Ribonucleotide reductases (RNRs) are essential enzymes that use radical-based chemistry to catalyze the reduction of ribonucleotides to deoxyribonucleotides. Anaerobic class III RNRs (NrdDs), the subject of this study, use an oxygen-sensitive glycyl radical cofactor and are members of the glycyl radical enzyme (GRE) family. The activity of NrdD enzymes can be allosterically up-regulated by ATP and down-regulated by dATP. We find that StNrdD’s regulatory “cone” domains adopt markedly different conformations depending on whether the activator ATP or the inhibitor dATP is bound and that these different conformations alternatively position an “active site flap” toward the active site (ATP-bound) or away (dATP-bound).

An x-ray structure of StNrdD bound to dATP was determined to 2.6-Å resolution by soaking WT-StNrdD crystals in 10 mM CTP and 10 mM dATP. Two dATP molecules are bound in the cone domain of StNrdD as was observed recently for PcNrdD and discussed in detail below. We find one dATP molecule bound in the canonical allosteric activity site (site 1) as first identified in EcRNR. The most unexpected feature of this dATP-bound StNrdD crystal structure is the asymmetric arrangement of the cone domains compared to the dimeric protein core. The cone domains, which form an antiparallel dimeric unit, are tilted so they contact only one side of the core fold, the side of the NrdD dimer that contains the opening to the chain B active site within the 10-stranded barrel. The chain B cone domain sits close to the top of the chain B barrel, not only burying a relatively large surface area near the barrel edge (525 Å2) but also making contacts with chain A across a chain A–chain B interface (left side of dimer in Fig. 2B). We find that the chain B cone domain is near the opening of the chain B barrel but the cone domain is rotated, such that the C terminus end of helix 4 is pointing away from the barrel opening (~180° away), pulling the connector in the opposite direction from the active site. Here, the C terminus of the cone domain helix 4 is pointing in the correct direction toward the chain A active site, but the chain A cone domain is sitting on the opposite side of the NrdD dimer from the barrel opening and is thus too far away for the connector to reach the active site (right). The asymmetry of the dATP-bound structure is therefore part of the mechanism of inhibition.

>[2x]MIILEKERVTVNPDIKVIKRDGRMVTFDSSKIYEAILKASETITPITPLIETKLEGIANRVVAEINDRFSHNIKIYEIQSIVEHELLEANEYAIAQEYINYRTKRDFERSQATDINFTINKLVNKDQAVVHENANKDSDLYNTQRDLTAGIVGKSVGLKMLPPHVANAHQKGDIHFHDLDYSPYTPMTNCCLIDFKGMLANGFKIGNAEVESPKSIQTATAQISQIIANVASSQYGGCTADRIDEFLAPYAELNYKKHLADAKEWVTEEKQEDYARAKTRKDIYDAMQSLEYEINTLFTSNGQTPFTSLGFGLGTNWFEREIQKAILQVRILGLGSEHRTAIFPKLIFTLKRGLNLEPNSPNYDIKQLALECATKRMYPDVLSYDKIIELTGSFKAPMGCRSFLQGWKDENGVEVNSGRMNLGVVTLNLPRIALESKGDQDKFWEIFEERMGIAKDALVYRVERVKEATPANAPILYQYGAFGQRLRKCDSVDQLFKHRRATVSLGYIGLYEVASVFYGSDWETNLEAKTFTLNIVKAMKNACESWSDEYDYHFSVYSTPSESLTDRFCRLDTEKFGVVTDITDKEYYTNSFHYDVRKNPTPFEKLEFEKDYPEAGATGGFIHYCEYPVLQQNPKALEAVWDFAYDRVGYLGTNTPIDKCYKCDFEGDFTPTERGFMCPNCGNTDPKTVDVVKRTCGYLGNPQARPMVKGRHKEISARVKHMNGSTIKYGGKHL>MAYSQGGGKKKVCYYYDGDIGNYYYGQGHPMKPHRIRMTHNLLLNYGLYRKMEIYRPHKATAEEMTKYHSDEYIKFLRSIRPDNMSEYSKQMQRFNVGEDCPVFDGLFEFCQLSTGGSVAGAVKLNRQQTDMAVNWAGGLHHAKKSEASGFCYVNDIVLAILELLKYHQRVLYIDIDIHHGDGVEEAFYTTDRVMTVSFHKYGEYFPGTGDLRDIGAGKGKYYAVNFPMRDGIDDESYGQIFKPIISKVMEMYQPSAVVLQCGADSLSGDRLGCFNLTVKGHAKCVEVVKTFNLPLLMLGGGGYTIRNVARCWTYETAVALDCEIPN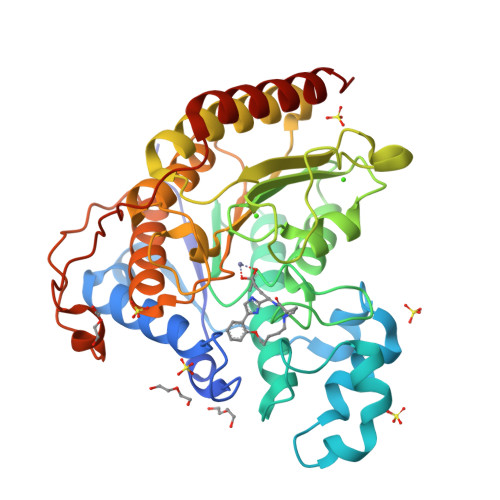ELPYNDYFEYFGPDFKLHISPSNMTNQNTPEYMEKIKQRLFENLRMLPH[3x]> MSSTPEKQTDPKAKANSIINAIPGNNILTKTGVLGTSAAAVIYAISNELYVINDESILLLTFLGFTGLVAKYLAPAYKDFADARMKKVSDVLNASRNKHVEAVKDRIDSVSQLQNVAETTKVLFDVS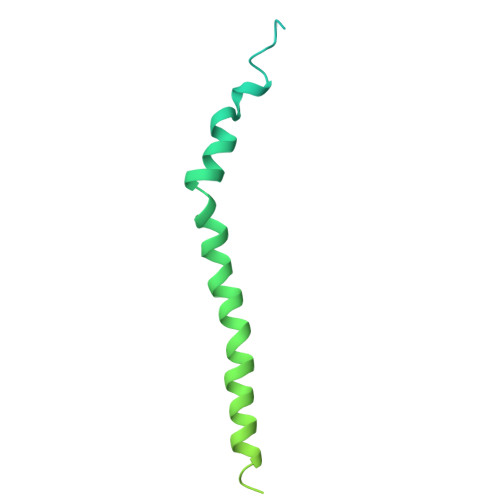KETVELESEAFELKQKVELAHEAKAVLDSWVRYEASLRQLEQRQLAKSVISRVQSELGNPKFQEKVLQQSISEIEQLLSKLK The ZIP family consists of divalent metal transporters that are ubiquitously expressed in all kingdoms of life, mediating metal flux into the cytoplasm from the extracellular milieu or from the intracellular organelles/vesicles. The prototypical ZIP from Bordetella bronchiseptica (BbZIP) is an elevator transporter, but how the metal substrate moves along the transport pathway and how the transporter changes conformation to allow alternating access remain to be elucidated. According to the proposed mechanism, a TM bundle composed of TM1/4/5/6 (the transport domain), carrying the metal substrate(s), moves vertically relative to the static scaffold domain composed of TM2/3/7/8 to achieve alternating access. Three metal binding sites have been identified in BbZIP, including the M1 and M2 sites at the transport site and the M3 site at the end of the metal release tunnel.

To fix the relative orientation of the two domains for structural characterization, A95 and A214 were substituted by cysteine residues, allowing chemical cross-linking between them as there is no endogenous cysteine residue in BbZIP. The inability to completely convert the A95C/A214C variant to the cross-linked form, presumably due to the highly dynamic nature of the transporter, led us to use mercury (Hg) as a cross-linker for structural study. After a brief treatment with EDTA and desalting, the Hg2+-cross-linked sample was crystallized in lipidic cubic phase under a Cd-free condition, yielding a structure of BbZIP in a new IFC conformation at 1.95 Å, the highest resolution for BbZIP to date. As expected, a Hg2+ is chelated by C95 from TM2 and C214 from TM5, locking the relative orientation between the transport and scaffold domains. Although the cross-linked A95C/A214C variant was briefly treated with EDTA and crystallized in a Cd2+-free buffer, the two tethered metal binding sites (M1 and M2) are still occupied by Cd2+. The coordination spheres of the bound Cd2+ are not significantly affected by the rigid-body hinge motion of the transport domain, but a chloride ion (Cl−) was found to coordinate with Cd2+ at the M1 site. Rather, the anion may assist metal release from the high-affinity transport site by neutralizing the charges on the cation and excluding the otherwise coordinating sulfur atom of M99 from the coordination sphere. The Cd2+ bound at the M3 site, with an occupancy of 0.84, is coordinated with two histidine residues (H149 and H151) from the intracellular loop 2 (hereafter IL2), D144 from TM3, E276 from TM7, and an ordered water molecule, forming a distorted octahedral coordination sphere. Although the IL2 of BbZIP was found to be severely disordered in the previous crystal structures, Cd2+ binding to the M3 site stabilizes the IL2 which folds into two short anti-parallel β-strands and forms hydrogen bonds with the rest of the protein.

> SHPLITLGLAASAAGVVLLLVAGIVNALTGENRVHVGYAVLGGAAGFAATALGALMALGLRAISARTQDAMLGFCAGMMLAASAFSLILPGLDAAGTIVGPGPAAAAVVALGLGLGVLLMLGLDYFTPHEHERTGHQGPEAARVNRVWLFVLTIILHNLPEGMAIGVSFATGDLRIGLPLTSAIAIQDVPEGLCVALALRAVGLPIGRAVLVAVASGLMEPLGALVGVGISSGFALAYPISMGLAAGAMIFVVSHEVIPETHRNGHETTATVGLMAGFALMMFLDTALG>[6x]MGHHHHHHHHHHSSGHIEGRHMTLTAREQRIQWFNHDRFGMFIHWGLYAIPARGEWVRSFERIPVEDYEKYFNSFNPVNYDPKAWAKAAKAAGMKYAVMTTKHHDGFCLFDSALTDYKATNTPAGRDLIREYADAFRAEGLKVGFYYSIIDWHHPDYPAYGDRQHPMRDNAEFKDRPQDFNRYLDYMHGQVKELLTNYGTIDVLWFDFSYEDMTGEKWKATELVKM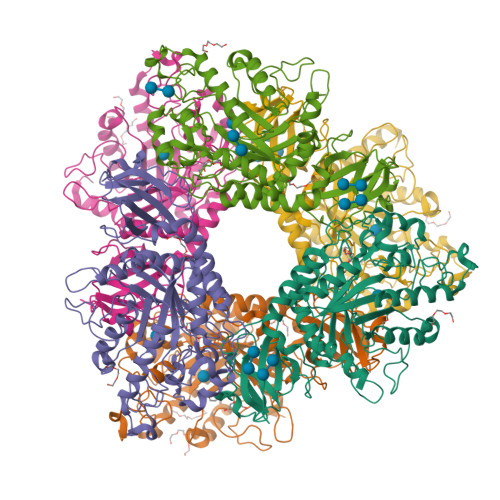IRELQPNVLIDNRLGGNIKAREPEIYAGDFASPEQLLPPHGIVNEDGKPLPWEACITLNHHWGYHAHDRDYKTPKQVVRGLVECVSKNGNMLLNVGPNAKGEIPQLSLDVLGEVGAWMRANGDSIYGCGAAALSKPEWGRYTQKGNKLYAHILDRGIGPIALQGLNGRVKEARLLADGAEVNIQTPWNAVDYPDYLFVNIPTAQLPDDFNTVIELTLEDAE>MNKRMNELVALLNRYATEYYTSDNPSVSDSEYDRLYRELVELETAYPEQVLADSPTHRVGGKVLDGFEKYSHQYPLYSLQDAFSRE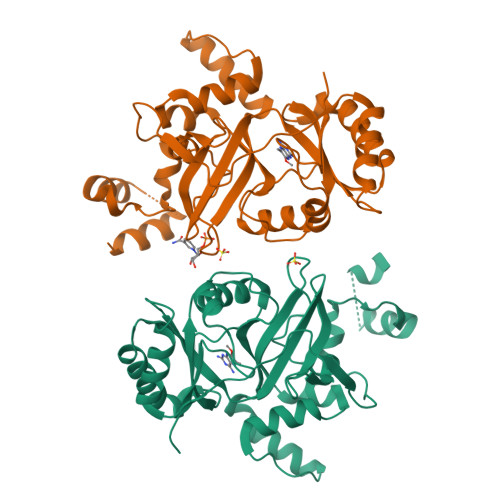ELDAFDARVRKEVAHPTYICELKIDGLSISLTYEKGILVAGVTRGDGSIGENITENLKRVKDIPLTLPEELDITVRGECYMPRASFDQVNQARQENGEPEFANPRNAAAGTLRQLDTAVVAKRNLATFLYQEASPSTRDSQEKGLKYLEQLGFVVNPKRILAENIDEIWNFIQEVGQERENLPYDIDGVVIKVNDLASQEELGFTVKAPKWAVAYKFPA[2x]> MELHQIRGCHKNDIELKKYNIGVAISLGNKWFSIDNIEKLVKWSLLHTKEYVIIYIADSIHGINLSVRNKLSDSHAEEVAIRYGRNLFIKIKERVSLSFSQDEQAKIIYATWSDIADSKYKEKVKYLYNLYDKNINFKNYIENFVKEWVSKEKRTFNNNEINKFGRYILEELPELMVQVKARGVLFEAFVYPYKTRITEFVGLLQKGEIFPEIKTNILDNHPKIFLEVRE

Cyclodipeptide synthases (CDPSs) use aminoacylated tRNA (aa-tRNA) substrates to form peptide bonds between two amino acids yielding a cyclic dipeptide product (CDP). ParaCDPS from Parabacteroides sp. 20_3 (GenBank: EFK64745.1) produces cyclo(His-Phe)8 whilst ParcuCDPS from Parcubacteria bacterium RAAC4_OD1_1 (GenBank: ETB63777.1) can synthesise both cyclo(His-Glu) and cyclo(His-Pro)9. ParcuCDPS belongs to the XYP sub-group of the CDPS family, characterised by the presence of 3 residues: X40 where X is a non-conserved residue, Y202, and P203 (numbering respective to AlbC). ParcuCDPS displays a Rossman-fold common throughout the CDPS family.

Inspired by HisRS and histidine recognition more generally, and by the only high resolution structure of a CDPS with a ligand bound, we systematically altered three unique residues in ParcuCDPS P1, which we hypothesised to be participating in crucial interactions with the polar side chain of histidine. We first designed Generation 1 containing seven P1 mutants (Y55F; Y55V; E174A; E174H; E174L; Y189F and Y189L), and these variants were cloned, expressed in E.coli, purified and used for activity assays. By mutating the P1 residues, the activity of the variants was vastly reduced with E174A and E174H incapable of tolerating histidine as a substrate. The impact of mutating Y55 carries more weight than Y189, suggesting it may directly interact with the histidine residue via a H-bond rather than adding to the polar surface. A similar pattern of residues interacting with the imidazole from histidine is seen in HisRS, in which two tyrosine and a glutamate residue mediate interactions with the nitrogen groups of histidine. Further investigation into the changes imposed by these mutants was performed by solving the crystal structures of a select few mutants containing changes to the active site or the pocket residues. The mutant structures were able to be solved using WT as a model and retained an equivalent fold to ParcuCDPS (Supplementary Notes 4 and 7 relating to Supplementary Figs. 13 and 14). Therefore, the disruption of activity is caused exclusively by the change in these few residues which appear important for the enzyme to produce a CDP.> MSQGRLEERLTISKRELARLLKELKKWSAPATVLLS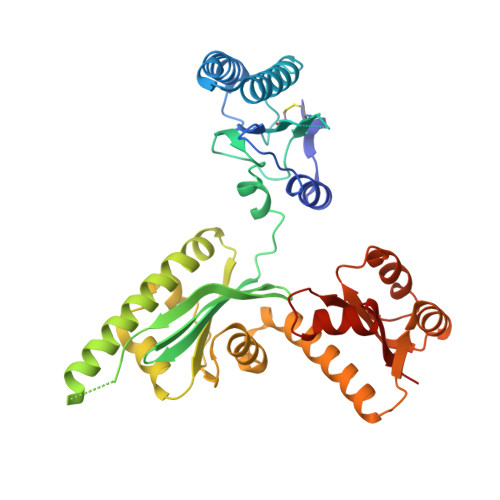LYIPPGRPLSDVMTLLRQEYSITDNIKLKRTRQAVKRALSAAMDRLQMLTSTPPNGLVLFCGEDMSTGKFECFMFSPPEPIRVFYYRTDKRFITDFLEDMVEDNNAIGIIIVERDQATIGLLKGARLEVLKELEGFVPGKHKMGGQSQRRYERIIEQMVDEFFKKVGEEASNLLVPLAEKGVLKGVIVAGPGLAKQEFVEGNYLDYRLKKILAPELVDVAYQGLQGLKEAVMKAEKVVEAQMYRDAVNAMEEFKLHLAKGTGMIVYGEKDVEAALEMGAVKTLLIHESREDLEEWVEKAKSSGAQVIVVPESLAEAEWFLKTFGGLAGILRFRISTV> MNRLPYFINYFFDTYLLINEDTPVGSSVTQLLARDLDNDPLVFGVVGEEASRFFAVESMTGVVWLRQPLDRETKSEFTVEFSVSDSQGVIKGSVNIQVGDVNDNAPRFHNQPYSVRIPENTPVGTPIFIVNATDPDQGAGGSVLYSFQPSSNFFTIDSGRGIVSVIR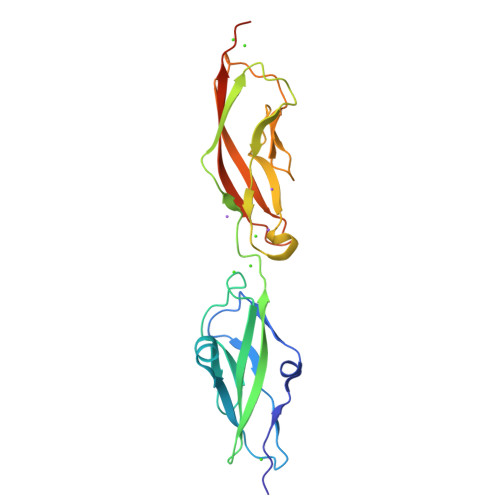ALDYEVTQAYQLQVNATDQDKTKPLSTLANLAITITDVQDMDPLEHHHHHH> NDPIANAVESAVSALADTTISRVTAANTTASTHSLGTGRVPALQAAETGASSNASDENLVETRCVMNRNGVNEASVEHFYSRAGLVGVVEVKDSGTSLDGYTVWPIDVMGFVQQRRKLELSTYMRFDAEFTFVSNLSNSTTPGMLLQYMYVPPGAPKPDGRKSYQWQTATNPSVFAKLSDPPPQVSVPFMSPATAYQWFYDGYPTFGEHKQATNLQYGQCPNNMMGHFAIRTVSESTTGKNVHVRVYMRIKHVRAWVPRPLRSQAYMVKNYPTYSQTITNTATDRASITTTDYEGGVPASPQRTS;> SPSVEACGYSDRVAQLTVGNSTITTQEAANIVLSYGEWPEYCPSTDATAVDKPTRPDVSVNRFYTLSTKSWKTESTGWYWKFPDVLNDTGVFGQNAQFHYLYRSGFCMHVQCNASKFHQGALLVAAIPEFVIAASSPATKPNGRGLYPDFAHTNPGKDGQEFRDPYVLDAGIPLSQALVFPHQWINLRTNNCATIIMPYVNALPFDSALNHSNFGLVVIPISPLKYCNGATTEVPVTLTIAPLNSEFSGLRQAIKQ;> GFPTELKPGTNQFLTTDDGTSPPILPGFEPTPLIHIPGEFTSLLDLCQIETILEVNNTTGTIGVSRLLIPVRAQNNVDQLCASFQVDPGRNGPWQSTMVGQICRYYTQWSGSLKVTFMFTGSFMATGKMLIAYTPPGSAQPATREAAMLGTHIVWDFGLQSSVTLVIPWISNTHFRAVKIGGVYDYYATGIVTIWYQTNFVVPPDTPTEANIIALGAAQK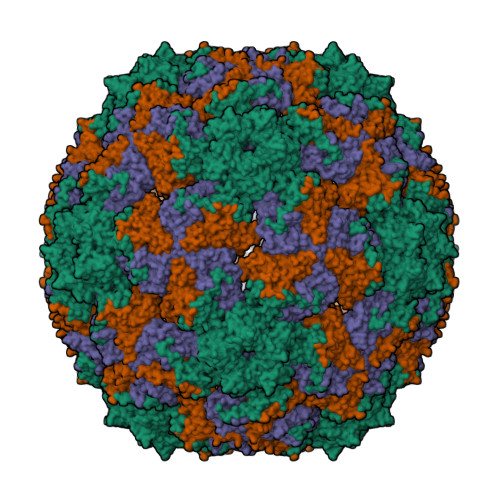NFTLKLCKDTDEIQQTAAYQ>[4x]SNAKIIGYARVSFNAQKDDLERQIQLIKSYAEENGWDIQILKDIGSGLNEKRKNYKKLLKMVM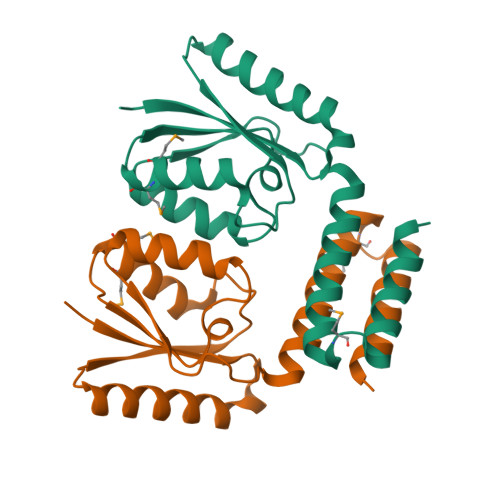NRKVEKVIIAYPDRLTRFGFETLKEFFKSYGTEIVIINKKHKTPQEELVEDLITIVSHFAGKLYGMHSHKYKKLTKTVKEIVREEDAKEKE>[4x]MSRPLLFALTALSLTAASLAHAADKKAADKPAPSAVSKADKALHDKFLTLDTHLDTPAHFGRPGWDIADHHEVEHDFSQVDL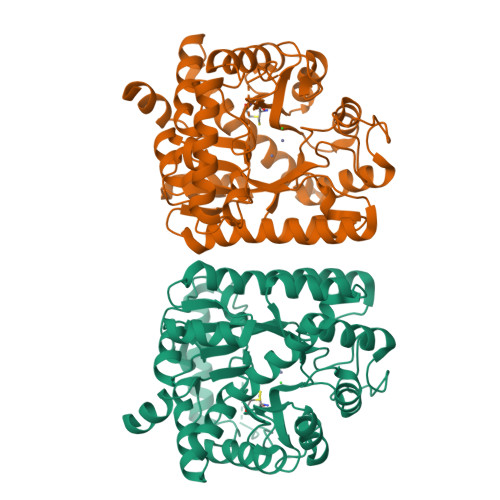PRMNQGGLDGGFFVVYIGQGELTEKGYTYARDYALHRTIEIREMLAANPDTFEMALTSDDARRIAKAGKKFAFVSMENSWPVGEDLSLVETFYKEGLRMAGPVHFRNNQLADSSTDPKGKIWNGYSPLGLRWLAEANRLGIVIDVSHASDDVVDQSVALSKAPIIASHSGPKAVYDHPRNLDDARLKKIADAGGAICINSIYLTDTTPSPERKAALEALGRAPDMKTATPEAVKAYADKRAAIDKAHPAARGDFDLYMKSMLHVLKVAGPKGVCVGADWDGGGGMDGFEDITDLPKITARLKAEGYSDADIEAIWSGNVLRIVDAAQAYAKSVTK methyl 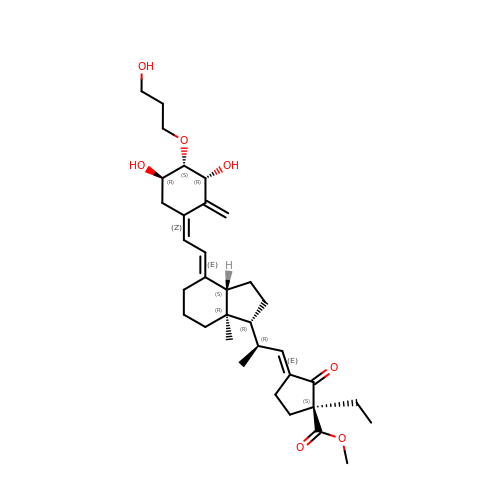(1S,3E)-3-{(2R)-2-[(1R,3aS,4E,7aR)-4-{(2Z)-2-[(3R,4S,5R)-3,5-dihydroxy-4-(3-hydroxypropoxy)-2-methylidenecyclohexylidene]ethylidene}-7a-methyloctahydro-1H-inden-1-yl]propylidene}-1-ethyl-2-oxocyclopentanecarboxylate (non-preferred name) | C34 H50 O7 | RRTPTPSZIBNWCN-ZZGOIYGKSA-N>GAMDTTYLTEEVKRGNIEKNVVATGSIESINTVDVGAQVSGKITKLYVKLGQQVKKGDLLAEIDPATYEADYQSAQANLASTQEQAQRYKLLVADQAVSKQQYADANAAYLQSKAAVEQARINLRYTKITSPIDGTVISTPVSEGQTVNSNQTTPTIIKVADLSKMRIKPEISEGDITKVKAGQDVTFTILSDNKTVYHAKIDSVDPATTTISDNSSSNSSSSGSSSSSGSSSSAVYYYANIIVENPEHVLRIGMTTENNIKIADVQNVLFIPNLAVQKQQDKYVVNVLNGNTTQEREIEIGVQN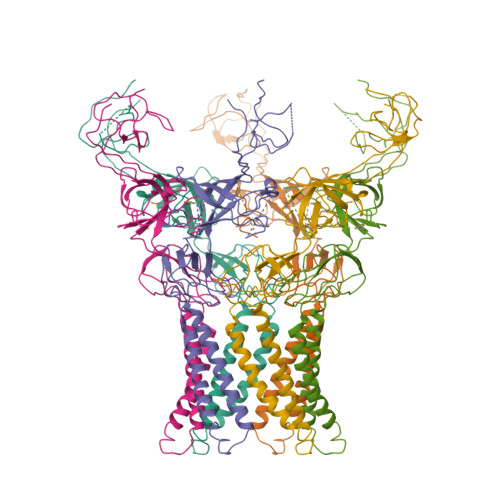DFQTEVKSGLTEGEKVVISQVAAGETFGDPDAPIIF[4x]Gram-positive pili differ from those of Gram-negative bacteria by the presence of covalently linked subunits containing a conserved LPXTG motif or a variant of it. In S. pneumoniae, the genes coding for the pilus are contained in a 12 Kb pathogenicity island (the rlrA islet), consisting of seven genes of which rrgA, rrgB, and rrgC encode LPXTG-containing proteins. Only RrgB is strictly necessary for the pilus formation while the other two are ancillary proteins. Here the crystal structure of the RrgBD2–D4 backbone subunit fitted into the EM reconstruction of the S. pneumoniae pilus reveals for the first time the polymeric architecture of a Gram-positive pilus indicating a head-to-tail organization of individual backbone subunits.

The fragment of RrgB designated RrgBD2-D4 (residues 184–627) was crystallized in three different crystal forms (in space groups P212121, P6122 and C2221). All the three forms of RrgBD2–D4 possess identical tertiary structure and all exhibited root mean square deviations (rmsds) with each other on aligned carbon alpha atoms of less than 7 Å. Each RrgBD2–D4 crystal form contained one molecule in the asymmetric unit, consisting of an elongated polypeptide (84 Å in length, 50 Å in width) made of three immunoglobulin-like domains (named D2, D3 and D4). The first 262 residues (184–446) form a dual domain (D2 and D3) made of two β-sandwiches of approximately 100 residues present in all crystal forms. The C-terminal 180 residues (446–627) form a third domain (D4) that contains an additional anti-parallel α-helical motif. All three domains D2, D3 and D4 are structurally homologous to each other, consisting of a pair of four-stranded β-sheets forming a β-sandwich configuration. We also find that each of the three crystallized domains of RrgB contains intra-molecular isopeptide bonds involving: Asn 318-Lys193 for D2; Asn 428-Lys349 for D3, and Asn 623-Lys453 for D4. The C-terminal immunoglobulin domain (D4) of the crystal structure matched well into the smaller globular density present below the groove with the core of seven β-strands placed internally the filament and the additional anti-parallel α-helical motif exposed on the surface. The fitting confirmed that pilus volume (∼155×e3 Å3) and dimensions (52 Å in width and 252 Å in length) could accommodate two RrgBD2–D4 molecules organized in a head-to-tail arrangement with rotations ranging between 17° and 22° along the vertical axis of the lower RrgBD2–D4 subunit in respect to the upper one.

> NTEAKPKIDKDFKGKANPDTPRVDKDTPVNHQVGDVVEYEIVTKIPALANYATANWSDRMTEGLAFNKGTVKVTVDDVALEAGDYALTEVATGFDLKLTDAGLAKVNDQNAEKTVKITYSATLNDKAIVEVPESNDVTFNYGNNPDHGNTPKPNKPNENGDLTLTKTWVDATGAPIPAGAEATFDLVNAQAGKVVQTVTLTTDKNTVTVNGLDKNTEYKFVERSIKGYSADYQEITTAGEIAVKNWKDENPKPLDPTEPKVVTYGKKFVKVNDKDNRLAGAEFVIANADNAGQYLARKADKVSQEEKQLVVTTKDALDRAVAAYNALTAQQQTQQEKEKVDKAQAAYNAAVIAANNAFEWVADKDNENVVKLVSDAQGRFEITGLLAGTYYLEETKQPAGYALLTSRQKFEVTATSYSATGQGIEYTAGSGKDDATKVVNKKIT> LPTSNPAQELEARQLGRTTRDDLINGNSASCADVIFIY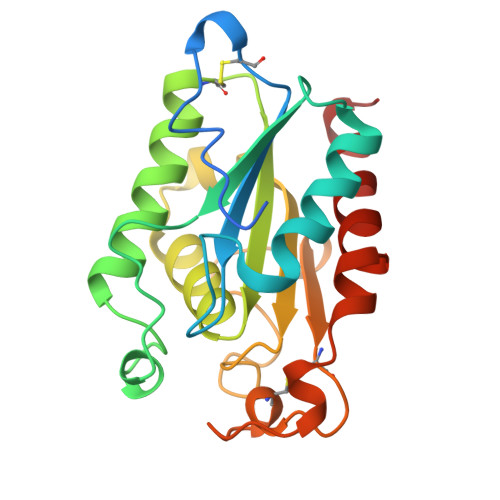ARGSTETGNLGTLGPSIASNLESAFGKDGVWIQGVGGAYRATLGDNFLPRGTSSAAIREMLGLFQQANTKCPDATLIAGGYSQGAALAAASIEDLDSAIRDKIAGTVLFGYTKNLQNRGRIPNYPADRTKVFCNTGDLVCTGSLIVAAPHLAYGPDARGPAPEFLIEKVRAVRGSA Gemin5 in the Survival Motor Neuron (SMN) complex serves as the RNA-binding protein to deliver small nuclear RNAs (snRNAs) to the small nuclear ribonucleoprotein Sm complex via its N-terminal WD40 domain. Additionally, the C-terminal region plays an important role in regulating RNA translation by directly binding to viral RNAs and cellular mRNAs. Here, we present the three-dimensional structure of the Gemin5 C-terminal region, which adopts a homodecamer architecture comprised of a dimer of pentamers. By structural analysis, mutagenesis, and RNA-binding assays, we find that the intact pentamer/decamer is critical for the Gemin5 C-terminal region to bind cognate RNA ligands and to regulate mRNA translation.

Symmetry expansion and focused refinement for the G5C protomer generated an overall map of 2.6 Å resolution. Consistent with the result from the SLS experiment, G5C forms a homodecamer with an MW of ~750 kDa. For each protomer, 531 out of 663 residues were unambiguously built, with several unresolved loop regions in the structure due to intrinsic flexibility. The G5C protomer is composed of 32 α-helices arranged in three regions. The N-terminal region of G5C consists of α1–α18, with α18 packing against α17 of the solved TPR domain (α1–α17) to form an extra TPR module. The middle region is composed of α19–α25. α22–α24 constitute a helix bundle, with α22 and α24 packing against α19–α21. The loop between α19 and α20 (aa 1133–1154) is invisible in the structure. α25 extends from α24 and connects the middle region to the C-terminal region. The C-terminal region consists of α26–α32 containing two helix bundles, α28–α29 and α26–α27–α31–α32. α30 is a short helix packing with α26, α28, and α29. The loops between α26 and α27 (aa 1294–1345) and between α28 and α29 (aa 1392–1429), as well as the last 12 C-terminal residues (aa 1497–1508), are invisible in the structure.

> GHMKKRKARSLLPLSTSLDHRSKEELHQDCLVLATAKHSRELNEDVSADVEERFHLGLFTDRATLYRMIDIEGKGHLENGHPELFHQLMLWKGDLKGVLQTAAERGELTDNLVAMAPAAGYHVWLWAVEAFAKQLCFQDQYVKAASHLLSIHKVYEAVELLKSNHFYREAIAIAKARLRPEDPVLKDLYLSWGTVLERDGHYAVAAKCYLGATCAYDAAKVLAKKGDAASLRTAAELAAIVGEDELSASLALRCAQELLLANNWVGAQEALQLHESLQGQRLVFCLLELLSRHLEEKQLSEGKSSSSYHTWNTGTEGPFVERVTAVWKSIFSLDTPEQYQEAFQKLQNIKYPSATNNTPAKQLLLHICHDLTLAVLSQQMASWDEAVQALLRAVVRSYDSGSFTIMQEVYSAFLPDGCDHLRDKLGDHQSPATPAFKSLEAFFLYGRLYEFWWSLSRPCPNSSVWVRAGHRTLSVEPSQQLDTASTEETDPETSQPEPNRPSELDLRLTEEGERMLSTFKELFSEKHASLQNSQRTVAEVQETLAEMIRQHQKSQLCKSTANGPDKNEPEVEAEQPLCSSQSQCKEEKNEPLSLPELTKRLTEANQRMAKFPESIKAWPFPDVLECCLVLLLIRSHFPGCLAQEMQQQAQELLQKYGNTKTYRRHCQTFCM>[2x]GUGCGAAGGGACG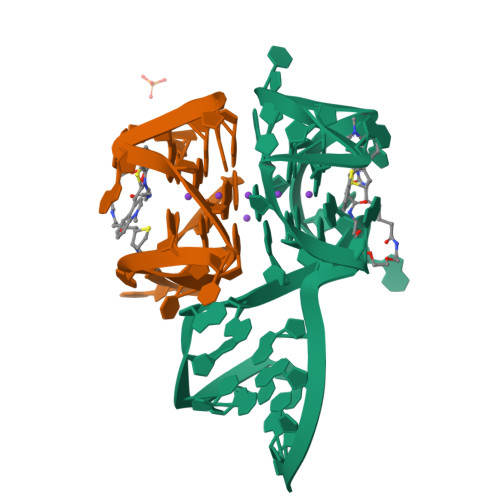GUGCGGAGAGGAGAGCAC>[20x]MKYDGSKLRIGILHARWNLEIIAALVAGAIKRLQEFGVKAENIIIETVPGSFELPYGSKLFVEKQKRLGKPLDAIIPIGVLIKGSTMHFEYICDSTTHQLMKLNFELGIPVIFGVLTCLTDEQAEARAGLIEGKMHNHGEDWGAAAVEMATKFNLEHHHHHH;>MGMKEKFVLIITHGDFGKGLLSGAEVIIGKQENVHTVGLNLGDNIEKVAKEVMRIIIAKLAEDK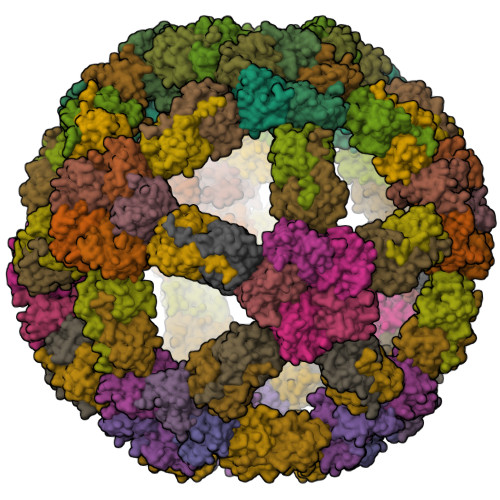EIIIVVDLFGGSPFNIALEMMKTFDVKVITGINMPMLVELLTSINVYDTTELLENISKIGKDGIKVIEKSSLKM[20x]1-[(3~{R})-3-[4-azanyl-3-(1~{H}-pyrrolo[2,3-b]pyridin-5-yl)pyrazolo[3,4-d]pyrimidin-1-yl]piperidin-1-yl]propan-1-one | C20 H22 N8 O | 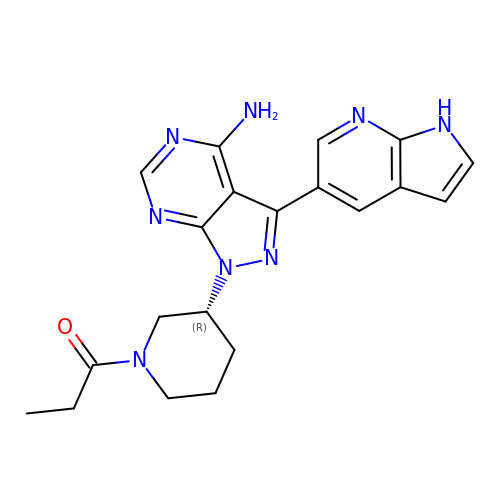BSJLZNJGXVKCML-CQSZACIVSA-N Fas-associated protein with death domain (FADD), procaspase-8, and cellular FLICE-inhibitory proteins (cFLIP) assemble through death-effector domains (DEDs), directing death receptor signaling towards cell survival or apoptosis. In this work, we present the crystal and cryo-EM structures of ternary FADD-Casp-8-cFLIP DED complexes, unveiling FADD-FADD, FADD-Casp-8, FADD-cFLIP, Casp-8-cFLIP, and cFLIP-cFLIP DED assemblies in a complex. The atomic coordinates depict how FADDDED and Casp-8tDED could assemble a helical 1:5 and 3:3 intermediate complexes, and how these FADD-Casp-8 intermediate complexes are targeted and capped by four cFLIPtDED molecules. The resultant helical Casp-8tDED-cFLIPtDED hetero-double layer appears to locally activate Casp-8.

To delve deeper into the assembly of the FADD-Casp-8-cFLIP complex, we conducted a study using wild-type (WT) full-length FADD, WT cFLIPtDED, and a full-length Casp-8 mutant with FGLG mutations, catalytic inactivity and processing deficiencies (F122G/L123G/C360A/D374A/D384A). This allowed us to reconstitute a ternary complex known as the FAFuL-C8FuL_FGLG_CADA-CF complex with an intact Casp-8 protease domain. To validate this observation, we produced a GraFix-stabilized version of the FAFuL-C8FuL_FGLG_CADA-CF complex and solved the cryo-EM structure at 3.7 Å resolution, named Complex B. Complex B confirmed the 3:3:4 model observed in Complex A, with invisible Casp-8 protease domain and FADD DD. Our triple-FADD complex structure unveils FADDDED-FADDDED and FADDDED-Casp-8tDED assemblies, by which three WT FADDDED molecules FAl, FAq, and FAr form a right-handed, type I interface-mediated trimer to interact with the left-handed Casp-8tDED trimer assembled by Casp-8tDED molecules C8a, C8b, and C8c. Notably, FADDDED interacts with the type Ib surface of C8tDED_FGLG DED2, although we introduced FGLG mutations on the type Ib surface, suggesting that the FL motif is dispensable for FADDDED-Casp-8tDED assembly. In addition, two FADDDED molecules FAq and FAr assemble like the Casp-8tDED molecule C8d in the single-FADD complex. Together they provide a type II and two type III surfaces, mimicking the type III-II-III CSS, for interaction with Casp-8tDED molecule C8c (d vs. 4e, f). In the 1:5:4 FAFuL_H9G-C8FGLG-CFH7G complex structure, three Casp-8tDED molecules C8c, C8d, and C8a provide, respectively, a type Ia, a type IIa, and a type IIIa surfaces, while FADDDED molecule FAl provides a type IIa and a type IIIa surfaces to complete the CBS to recruit cFLIPtDED_H7G molecule CFk. A similar CBS, which recruits WT cFLIPtDED molecule CFk (CFk-binding CBS), was also found in the 3:3:4 FAFuL-C8FuL_FGLG_CADA-CF complex structure, although Casp-8tDED C8d is replaced by two WT FADDDED molecules FAr and FAq (Fig. 5c vs 5e). In fact, the triple-FADD structure demonstrates that FADD can physically impede Casp-8 filamentation at the upper end.

>MDFSRNLYDIGEQLDSEDLASLKFLSLDYIPQRKQEPIKDALMLFQRLQEKRMLEESNLSFLKELLFRINRLDLLITYLNTRKEEMERELQTPGRAQISAYRVMLYQISEEVSRSELRSFKGGLQEEISKCKLDDDMNLLDIFIEMEKRVILGEGKLDILKRVCAQINKSLLKIINDYEEFSKERSSSLEGSPDEFSNGEELCGVMTISDSPREQDSESQTLDKVYQMKSKPRGYCLIINNHNFAKAREKVPKLHSIRDRNGTHLDAGALTTTFEELHFEIKPHDDCTVEQIYEILKIYQLMDHSNMDCFICCILSHGDKGIIYGTDGQEAPIYELTSQFTGLKCPSLAGKPKVFFIQAAQGDNYQKGIPVETASEEQPYLEMALSSPQTRYIPDEADFLLGMATVNNCVSYRNPAEGTWYIQSLCQSLRERCPRGDDILTILTEVNYEVSNKDDKKNMGKQMPQPTFTLRKKLVFPSD[3x];>MSAEVIHQVEEALDTDEKEMLLFLCRDVAIDVVPPNVRDLLDILRERGKLSVGDLAELLYRVRRFDLLKRILKMDRKAVETHLLRNPHLVSDYRVLMAEIGEDLDKSDVSSLIFLMKDYMGRGKISKEKSFLDLVVELEKLNLVAPDQLDLLEKCLKNIHRIDLKTKIQKYKQSVQGAGTS[4x];>[3x]MDPFLVLLHSVSSSLSSSELTELKFLCLGRVGKRKLERVQSGLDLFSMLLEQNDLEPGHTELLRELLASLRRHDLLRRVDDFEAGAAAGAAPGEEDLCAAFNVICDNVGKDWRRLARQLKVSDTKIDSIEDRYPRNLTERVRESLRIWKNTEKENATVAHLVGALRSCQMNLVADLVQEVQQARDLQNRSGAMSPMSWNSDASTSEASLEHHHHHH>GPLGSMKTVFSPLHSRRHVKTELDGG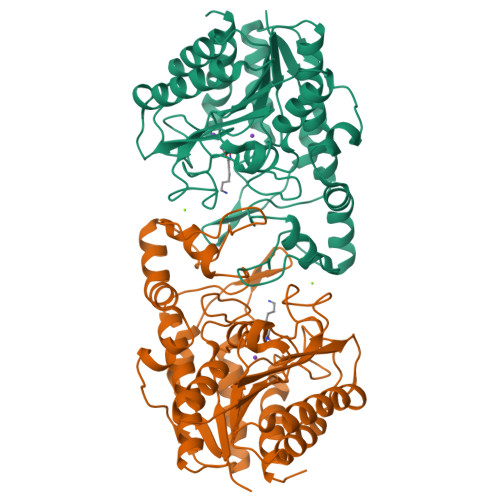LLIEPHEKPSRAETILARVKDQALGEILEPEEFGLGPVKRVHTADYVSFLETCWDEWVAAGKRGEAIPTFWVGRGMRARLPKDIDGRLGYYSLGADTSISDGTWEAARASANVALTAQKLVAEGERAAFALCRPPGHHAHADVFGGYCFFNNAAIAAQAFRDQGYGKVAVLDVDFHHGNGTQAIFYDRSDVLTISLHGDPDLVFPHFLGFEDETGEGDGEAYNLNIVFPPDTPFSIWSQGLEKACERIRTFAPDALVVALGVDTFEEDPISFFKLTSGDYLKLGKRLEQLGLPTVFTMEGGYDVDAIGVNAVNVMQGFEGKS[8x]> MGSHHHHHHSQDSVTIFILSVIHVKPPFKLKRKFQNNPHYEKEMRRQLKMQEDGINKLTVFEWLTNRKTFREKGRLSSQTAQND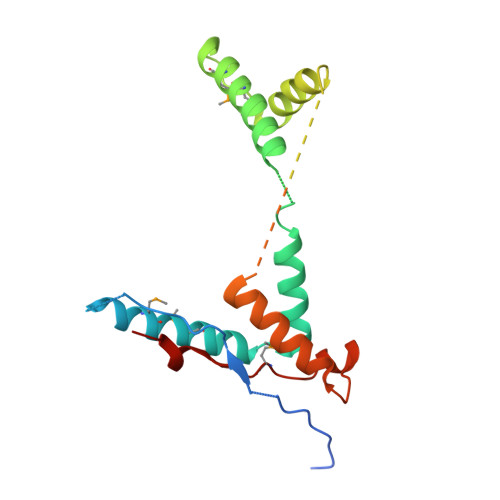ARDAYKRRKMFDYMLLSAENFKYDEITKKVEDELSSLAALHNPDQIAGGNFDDVTAMGDKRINSSIGSQWGTKDKGRAQNLEDELLKVLEGPPKIDEEQQKYIKMNVIFAEDLEIIK3,5-dichloro-2-hydroxybenzoic acid | C7 H4 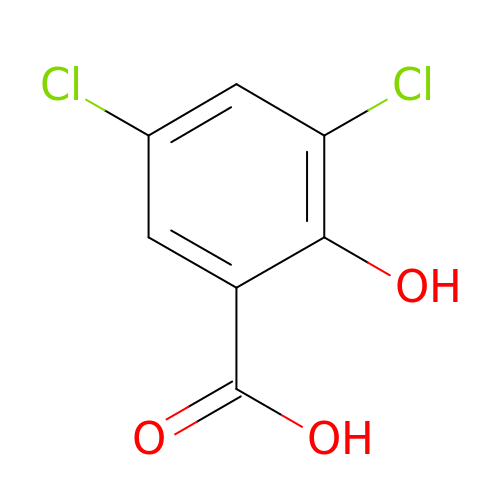Cl2 O3 | CNJGWCQEGROXEE-UHFFFAOYSA-N>MVHHHHHHLLVPRGSKIEEVKSTTKTQRIASHSHVKGLGLDESGLAKQAASGLVGQENAREACGVIVELIKSKKMAGRAVLLAGPPGTGKTALALAIAQELGSKVPFCPMVGSEVYSTEIKKTEVLMENFRRAIGLRIKEGPPGIIQDVTLHDLDVANARPQGGQDILSMMGQLMKPKKTEITDKLRGEINKVVNKYIDQGIAELVPGVLFVDEVHMLDIECFTYLHRALESSIAPIVIFASNRGNCVIRGTEDITSPHGIPLDLLDRVMIIRTMLYTPQEMKQIIKIRAQTEGINISEEALNHLGEIGTKTTLRYSVQLLTPANLLAKINGKDSIEKEHVEEISELFYDAKSSAKILADQQDKYMK[3x];>[3x]MDYKDDDDKENLYFQGATVTATTKVPEIRDVTRIERIGAHSHIRGLGLDDALEPRQASQGMVGQLAARRAAGVVLEMIREGKIAGRAVLIAGQPGTGKTAIAMGMAQALGPDTPFTAIAGSEIFSLEMSKTEALTQAFRRSIGVRIKEGPPGVVHTVSLHEIDVINSRTQGFLALFSGDTGEIKSEVREQINAKVAEWREEGKAEIIPGVLFIDEVHMLDIESFSFLNRALESDMAPVLIMATNRGITRIRGTSYQSPHGIPID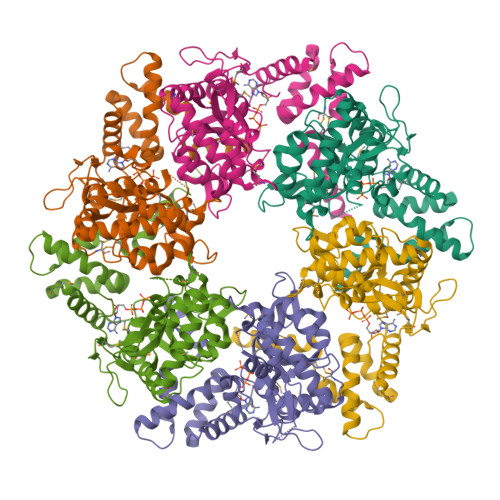LLDRLLIVSTTPYSEKDTKQILRIRCEEEDVEMSEDAYTVLTRIGLETSLRYAIQLITAASLVCRKRKGTEVQVDDIKRVYSLFLDESRSTQYMKEYQDAFLFNELKGETMDTS>[2x]GSEAAGGEQRELLIQRLRAAVHYTTGALAQDVAEDKGVLFSKQTVAAISEITFRQAENFARDLEMFARHAKRSTITSEDVKLLARRSNSLLKYITQKSDELASSNME;>[2x]GYEEREGGFRKETVERLLRLHFRDGRTRVNGDALLLMAELLKVFVREAAARAARQAQAEDLEKVDIEHVEKVLPQLLLDFV;> GRSLHHKSALFSCVTDPKEMHCHENWSLSPEEFEIWDRLYRLKENDGVKEPILPHTRFETLENLDKTSKPEEEAAHKLSLSEWSIWQSRPFPTSMVDHSDRCYHFISVMELIEVMRQEQGDCSYELELQPHLRIEDIHVRRNKGHLSP

FANCM is involved in eukaryotic DNA-damage recognition and activates the Fanconi anemia (FA) pathway through complex formation. MHF is one of the FANCM-associating components and contains a histone-fold DNA-binding domain. The FANCM-associated histone-fold protein (MHF) 1/2 complex (also known as CENP-S/CENP-X) associates with the conserved region of FANCM immediately after the helicase domain to form a FANCM–MHF complex. MHF stabilizes FANCM and promotes its DNA-binding activity.

Unexpectedly, structure determination revealed that one of the crystals contained the FANCM–MHF complex but that the other two contained the MHF complex without FANCM. It contained one FANCM–MHF heteropentamer in the asymmetric unit, with FANCM asymmetrically bound to the MHF heterotetramer. We could model most of MHF and FANCM except for the N-terminal 13 residues. FANCM interacts with MHF through an extensive surface area of more than 5000 Å2. The interaction is formed by hydrogen bonding, salt bridges and hydrophobic interactions. Mapping of MHF hydrophobicity indicates that the interface is more hydrophobic than the other regions. In the current chicken FANCM–MHF crystal structure, the corresponding cysteine residue (Cys759) does not coordinate an ion. On the other hand, Cys670, Cys679 and Cys779 are exposed to solvent; in particular, Cys670 is in the disordered region and may be sensitive to oxidation.>MTDMNILDLFLKASLLVKLIMLILIGFSIASWAIIIQRTRILNAAAREAEAFEDKFWSGIELSRLYQESQGKRDNLTGSEQIFYSGFKEFVRLHRANSHAPEAVVEGASRAMRISMNRELENLETHIPFLGTVGSISPYIGLFGTVWGIMHAFIALGAVKQATLQMVAPGIAEALIATAIGLFAAIPAVMAYNRLNQRVNKLELNYDNFMEEFTAILHRQAFTVSESNKG[5x];>[2x]MGSWSHPQFEKGSSKATEQNDKLKRAIIISAVLHVILFAALIWSSFDENIEASAGGGGGSSIDAVMVDSGAVVEQYKRMQSQESSAKRSDEQRKMKEQQAAEELREKQAAEQERLKQLEKERLAAQEQKKQAEEAAKQAELKQKQAEEAAAKAAADAKAKAEADAKAAEEAAKKAAADAKKKAEAEAAKAAAEAQKKAEAAAAALKKKAEAAEAAAAEARKKAATEAAEKAKAEAEKKAAAEKAAADKKAAAEKAAADKKAAEKAAAEKAAADKKAAAEKAAADKKAAAAKAAAEKAAAAKAAAEADDIFGELSSGKNAPKTGGGAKGNNASPAGSGNTKNNGASGADINNYAGQIKSAIESKFYDASSYAGKTCTLRIKLAPDGMLLDIKPEGGDPALCQAALAAAKLAKIPKPPSQAVYEVFKNAPLDFKP;>[2x]MARARGRGRRDLKSEINIVPLLDVLLVLLLIFMATAPIITQSVEVDLPDATESQAVSSNDNPPVIVEVSGIGQYTVVVEKDRLERLPPEQVVAEVSSRFKANPKTVFLIGGAKDVPYDEIIKALNLLHSAGVKSVGLMTQPI

The Ton and Tol systems are sophisticated molecular machineries essential for virulence and survival of Gram-negative bacteria. Both systems rely on the proton gradient at the inner membrane to produce force and movement that are transmitted to target proteins associated with the outer membrane. Ton is involved in the uptake of essential nutrients such as siderophore-iron, vitamin B12 and carbohydrates, while Tol maintains outer membrane integrity and plays an active role in cell division. We have solved the high-resolution structures of the E. coli TonB-ExbB-ExbD and TolA-TolQ-TolR complexes, revealing the inner membrane embedded engine parts of the Ton and Tol systems, and showing how TonB and TolA interact with the ExbBD and TolQR subcomplexes.

We hypothesized that the elongated periplasmic domain of TolA was the main source of heterogeneity, and we engineered a construct with a TEV proteolysis site between Ile50 and Asp51. The stoichiometry of the TolATEVQR complex is two TolA, five TolQ and two TolR. TolAQR is a pentamer of TolQ, a dimer of TolR inside the TolQ pentamer, and two TM of TolA binding at the periphery of the pentamer. The structure reveals most of the TolQ subunit (residues 2-225), the N-terminus and TM of TolR (8-40) and the TM of TolA (4-34). The periplasmic domains of both TolA and TolR were not visible, suggesting these regions are flexible. TolA TM is a 40 Å long, straight α-helix, tilted 20° relative to the perpendicular axis to the membrane plane, in the opposite direction of TolQ α−2 TM. The highly conserved and essential TolA His2221 makes multiple contacts with TolQ Ser28, Trp32 and Ile29. There are two TolA in the TolAQR complex, which are bound to TolQ chains C and E. Comparison of the two structures shows significant displacement of the cytoplasmic regions of TolQ chains A, B and C, whereas the structures of the transmembrane and periplasmic regions are virtually identical. The two structures of TolAQR described in this report show that TolQ can adopt different conformations, with a high degree of flexibility between the cytoplasmic and TM domains.>[6x]MPKPYVAINMAELKNEPKTFEMFASVGPKVCMVTARHPGFVGFQNHIQIGILPFGNRYGGAKMDMTKESSTVRVLQYTFWKDWKDHDEMHRQNWSYLFRLCYSCASQMIWGPWEPIYEIIYANMPINTEMTDFTAVVGKKFAEGKPLDIPVISQPYGKRVVAFAEHSVIPGKEKQFEDAIVRTLEML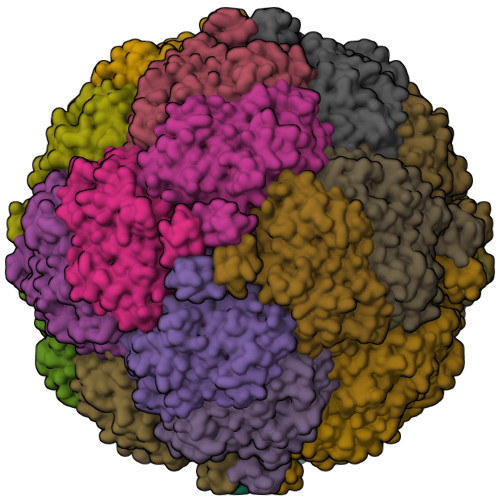KKAPGFLGAMVLKEIGVSGIGSMQFGAKGFHQVLENPGSLEPDPNNVMYSVPEAKNTPQQYIVHVEWANTDALMFGMGRVLLYPELRQVHDEVLDTLVYGPYIRILNPMMEGTFWREYLNENAWRHPQFGG> KNPKSDKFKVKRFHHIEFWCGDATNVARRFSWGLGMRFSAKSDLSTGNMVHASYLLTSGDLRFLFTAPYSPSLSAGEIKPTTTASIPSFDHGSCRSFFSSHGLGVRAVAIEVEDAESAFSISVANGAIPSSPPIVLNEAVTIAEVKLYGDVVLRYVSYKAEDTEKSEFLPGFERVEDASSFPLDYGIRRL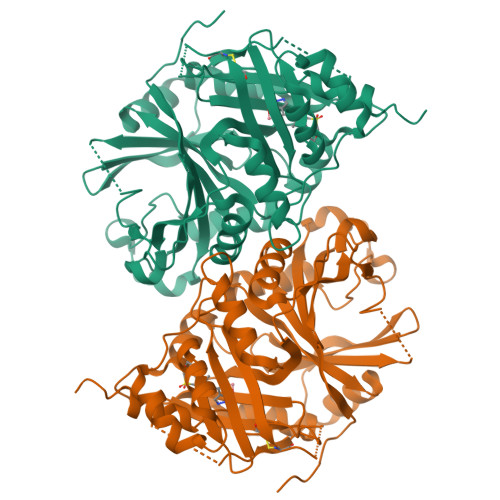DHAVGNVPELGPALTYVAGFTGFHQFAEFTADDVGTAESGLNSAVLASNDEMVLLPINEPVHGTKRKSQIQTYLEHNEGAGLQHLALMSEDIFRTLREMRKRSSIGGFDFMPSPPPTYYQNLKKRVGDVLSDDQIKECEELGILVDRDDQGTLLQIFTKPLGDRPTIFIEIIQRVGCMMKDEEGKAYQSGGCGGFGKGNFSELFKSIEEYE> MLMKRLFAASLMLAFSSVSSVRAEEAVKPGAP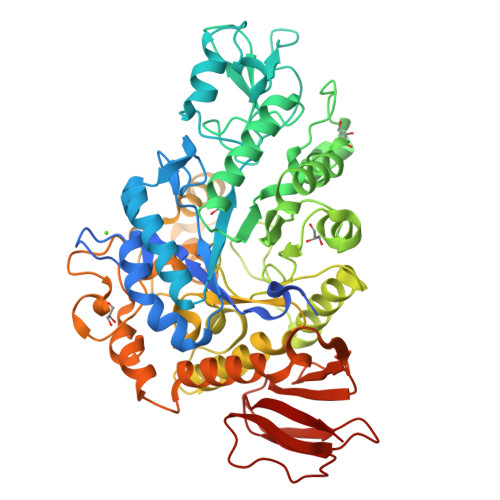WWKSAVFYQVYPRSFKDTNGDGIGDFKGLTEKLDYLKGLGIDAIWINPHYASPNTDNGYDISDYREVMKEYGTMEDFDRLMAELKKRGMRLMVDVVINHSSDQHEWFKSSRASKDNPYRDYYFWRDGKDGHEPNNYPSFFGGSAWEKDPVTGQYYLHYFGRQQPDLNWDTPKLREELYAMLRFWLDKGVSGMRFDTVATYSKTPGFPDLTPEQMKNFAEAYTQGPNLHRYLQEMHEKVFDHYDAVTAGEIFGAPLNQVPLFIDSRRKELDMAFTFDLICYDRALDRWHTIPRTLADFRQTIDKVDAIAGEYGWNTFFLGNHDNPRAVSHFGDDRPQWREASAKALATVTLTQRGTPFIFQGDELGMTNYPFKTLQDFDDIEVKGFFQDYVETGKATAEELLTNVALTSRDNARTPFQWDDSANAGFTTGKPWLKVNPNYTEINAAREIGDPKSVYSFYRNLISIRHETPALSTGSYRDIDPSNADVYAYTRSQDGETYLVVVNFKAEPRSFTLPDGMHIAETLIESSSPAAPAAGAASLELQPWQSGIYKVK> LPESVDWRAKGAVTPVKHQGYCESCWAFSTVATVEGINKIKTGNLVELSEQELVDCDLQSYGCNRGYQSTSLQYVAQNGIHLRAKYPYIAKQQTCRANQVGGPKVKTNGVGRVQSNNEGSLLNAIAHQPVSVVVESAGRDFQNYKGGIFEGSCGTKVDHAVTAVGYGKSGGKGYILIKNSWGPGWGENGYIRIRRASGNSPG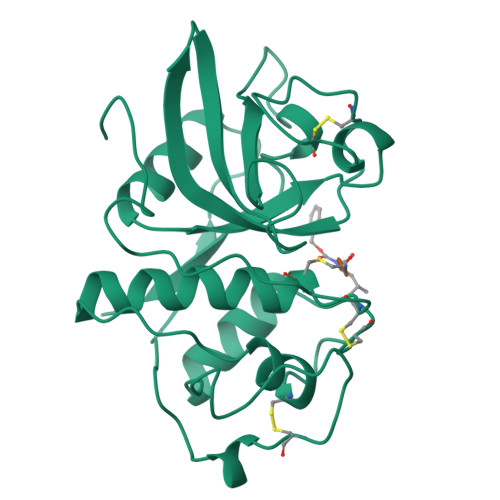VCGVYRSSYYPIKN>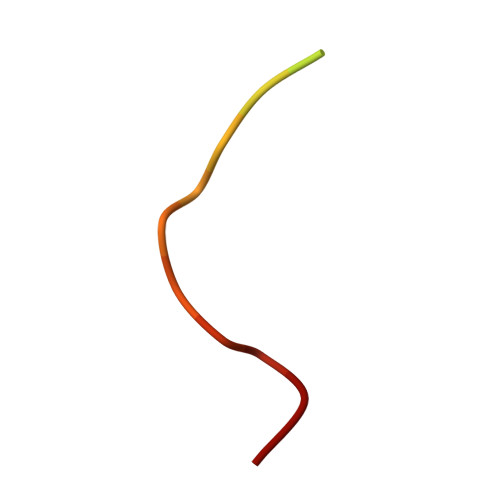 MKRARPSGDTFNPVYPYDT> MDHAPERFDATPPAGEPDRPALGVLELTSIARGITVADAALKRAPSLLLMSRPVSSGKHLLMMRGQVAEVEESMIAA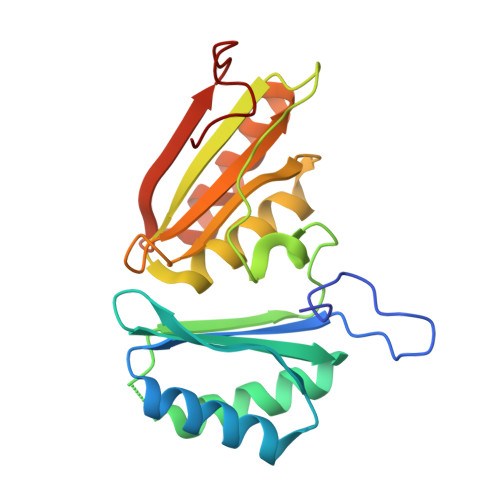REIAGAGSGALLDELELPYAHEQLWRFLDAPVVADAWEEDTESVIIVETATVCAAIDSADAALKTAPVVLRDMRLAIGIAGKAFFTLTGELADVEAAAEVVRERCGARLLELACIARPVDELRGRLFF>[4x]MSLEKQKGLAIITGASQGIGAVIAAGLATDGYRVVLIARSKQNLEKVHDEIMRSNKHVQEPIVLPLDITDCTKADTEIKDIHQKYGAVDILVNAAAMFMDGSLS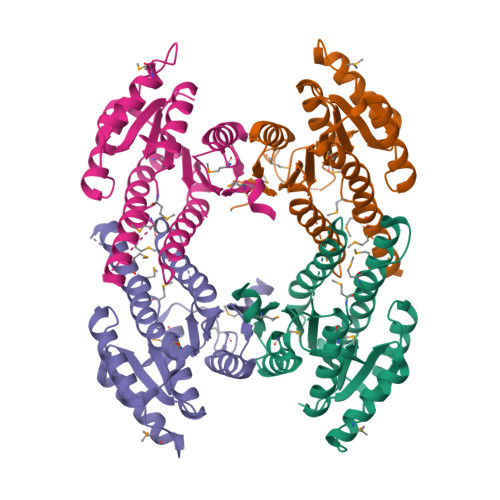EPVDNFRKIMEINVIAQYGILKTVTEIMKVQKNGYIFNVASRAAKYGFADGGIYGSTKFALLGLAESLYRELAPLGIRVTTLCPGWVNTDMAKKAGTPFKDEEMIQPDDLLNTIRCLLNLSENVCIKDIVFEMKKSIIEGHHHHHH>[10x]NKGSIEGREPAVYFKEQFLDGDGWTSRWIESKHKSDFGKFVLSSGKFYGDEEKDKGLQTSQKARFYALSASFEPFSNKGQTLVVQFTVKHEQNIDCGGGYVKLFPNSLDQTDMHGDSEYNIMFGPDICGPGTKKVHVIFNYKGKNVLINKDIRCKDDEFTHLYTLIVRPDNTYEVKIDNSQVESGSLEDDWDFLPGSGDPSIYAYDNFGVLGLDLWQVKSGTIFDNFLITNDEAYAEEFGNETWGVTKAAEKQMKDKQDEEQRLK

Calreticulin (CRT) is a 46 kDa soluble multifunctional protein that was initially identified as an endoplasmic reticulum (ER) chaperone for monoglycosylated proteins and is also involved in Ca2+ regulation. Similar to its ER membrane homologue calnexin (CNX) ectodomain, CRT is composed of a globular domain, into which a flexible arm-like P (proline-rich) domain is inserted. The globular domain is made up of seven concave and six convex β-sheets forming a legume lectin fold. We have investigated the CRTs of two distinct parasites, Trypanosoma cruzi (TcCRT) and Entamoeba histolytica (EhCRT), for which a pathogenic role has been proposed.

The purpose of this HsCRT mutant was to disrupt an ionic bond observed in all previous crystal packing(s) that stabilizes CRT molecular arrays. As expected from the mutation design, a new crystal form has been obtained, with ten independent copies now present in the asymmetric unit. The residues of the conserved lectin site (analysed below in §3.3) do not participate in the packing interactions in this new crystal form. Compared with the previous native HsCRT structure, the largest deviation was observed for its N-terminal extension, which, in the absence of interaction with a neighbouring lectin site, is more flexible and found in different orientations up to Val21. The part of the junction and linker region (LPGSGD) which was not initially defined in the wild-type (wt) model has been rebuilt in most of the copies. The final average root-mean-square deviation (r.m.s.d.) between the wt HsCRT structure and the different HsCRT D71K copies is very small (0.3 Å).>GMNPAAEAEFNILLATDSYKVTHYKQYPPNTSKVYSYFECREKKTENSKLRKVKYEETVFYGLQYILNKYLKGKVVTKEKIQEAKDVYKEHFQDDVFNEKGWNYILEKYDGHLPIEIKAVPEGFVIPRGNVLFTVENTDPECYWLTNWIETILVQSWYPITVATNSREQKKILAKYLLETSGNLDGLEYKLHDFGYRGVSSQETAGIGASAHLVNFKGTDTVAGLALIKKYYGTKDPVPGYSVPAAEHSTITAWGKDHEKDAFEHIVTQFSSVPVSVVSDSYDIYNACEKIWGEDLRHLIVSRSTQAPLIIRPDSGNPLDTVLKVLEILGKKFPVTENSKGYKLLPPYLRVIQGDGVDINTLQEIVEGMKQKMWSIENIAFGSGGGLLQKLTRDLLNC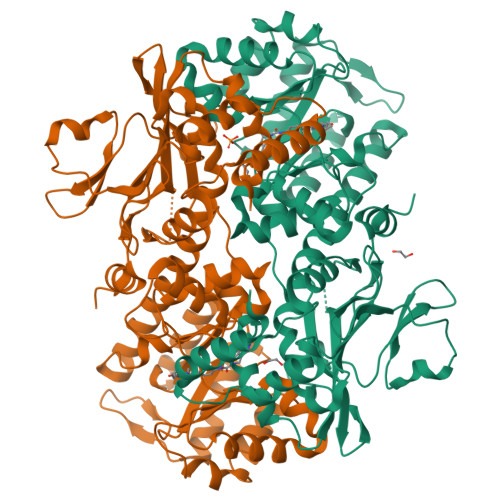SFKCSYVVTNGLGINVFKDPVADPNKRSKKGRLSLHRTPAGNFVTLEEGKGDLEEYGQDLLHTVFKNGKVTKSYSFDEIRKNAQLNIELEAAHH[4x]> QIYSARYSGVDVYEFIHSTGSIMKRKKDDWVNATHILKAANFAKAKRTRILEKEVLKETHE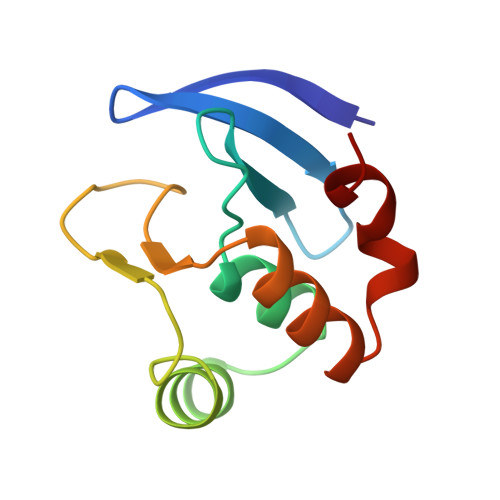KVQGGFGKYQGTWVPLNIAKQLAEKFSVYDQLKPLFDF> GPLGSQSSCKAKVANIIAEVAKNEFMRIPCVDAGLISPLVQLLNSKDQEVLLQTGRALGNICYDSHSLQAQLINMGVIPTLVKLLGIHCQNAALTEMCLVAFGNLAELESSKEQFASTNIAEELVKLFKKQIEHDKREMIFEVLAPLAENDAIKLQLVEAGLVECLLEIVQQKVDSDKEDDITELKTGSDLMVLLLLGDESMQKLFEGGKGSVFQRVLSWIPSNNHQLQLAGALAIANFARNDANCIHM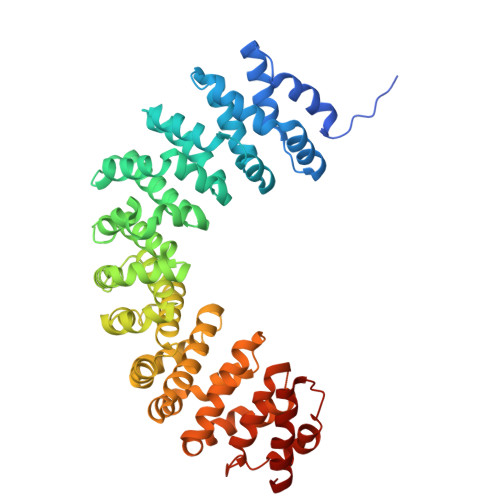VDNGIVEKLMDLLDRHVEDGNVTVQHAALSALRNLAIPVINKAKMLSAGVTEAVLKFLKSEMPPVQFKLLGTLRMLIDAQAEAAEQLGKNVKLVERLVEWCEAKDHAGVMGESNRLLSALIRHSKSKDVIKTIVQSGGIKHLVTMATSEHVIMQNEALVALALIAALELGTAEKDLESAKLVQILHRLLADERSAPEIKYNSMVLICALMGSECLHKEVQDLAFLDVVSKLRSHENKSVAQQASLTEQRLTVES> FHLTTRNGEPHMIVSRQEKGKSLLFKTEDGVNMCTLMAMDLGELCEDTITYKCPFLKQNEPEDIDCWCNSTSTWVTYGTCTTTGEHRREKRSVALVPHVGMGLETRTETWMSSEGAWKHAQRIETWILRHPGF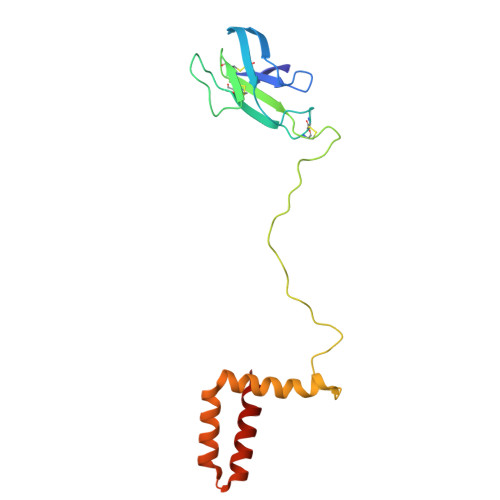TIMAAILAYTIGTTHFQRALIFILLTAVAPSMT>MRTRSQVWAQKAYEKVREAAKGEGRGEYRDMALKLPVLVRQAGLSQALAFVDSRGKEAHKALGNDLAQVLGYRDLRELAEAAREAELLQYLRLTREVLAAA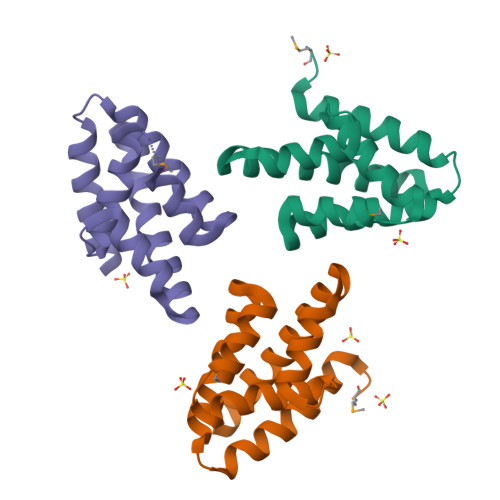EWFKRFAQALIEE[6x]> MNNGEGEVMDLRDIDLNLLVVFNQLLLDRSVSTAGEKLGLTQPAVSNSLKRLRTALNDDLFLRTSKGMEPTPYALHLAEPVIYALNTLQTALTTRNSFDPFASTRTFNLAMTDIGEMYFMPPLMEALAQRAPHIQISTLRPNAGNLKEDMESGAVDLALGLLPELQTGFFQRRLFRHRYVCMFRKDHPSAKSPMSLKQFSELEHVGVVALNTGHGEVDGLLERAGIKRRMRLVVPHFIAIGPILHSTDLIATVPQRFAVRCEVPFGLTT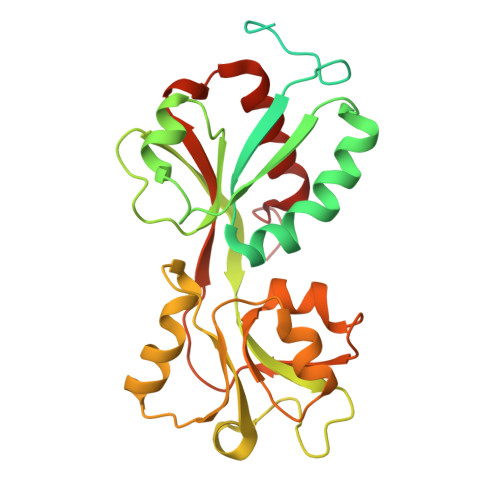SPHPAKLPDIAINLFWHAKYNRDPGNMWLRQLFVELFSEAHHHHHH>HHHHHHENLYFQSMAVSPSPLRIFTAGGTIDKDARLEENGLVVGDPFVAEVLKTARLAGAVSIVALSRKDSLDFTEADREAIGRAVGQAVEDHILLTHGTDTMVETARYLGGLPELAGKTVVLSGAMVPGRVGGSDAAFNIGFACAAALMLAPGVYIAMHGKVFDPAKTRKNRGLGRFEPIDDQE[4x]

L‐Asparaginases (ASNases) catalyze the hydrolysis of L‐Asn to L‐Asp and ammonia. In contrast, the chain of ASNase from Rhodospirillum rubrum, reported here and referred to as RrA, consists of only 172 amino acid residues. RrA is homologous to the N‐terminal domain of typical bacterial class 1 ASNases and exhibits millimolar affinity for L‐Asn. Crystal structures of the wild‐type RrA, both with and without bound L‐Asp, as well as structures of several RrA mutants, reveal topologically unique tetramers.

Based on the previously published results for typical class 1 ASNases (Derst et al., 1994; Schalk et al., 2016), we tested two mutants, RrA(Y21A) and RrA(Y21F). RrA(Y21A) without added L‐Asp was disordered in the region of residues 22–26 and the active site contained a mostly disordered HEPES molecule contributed by the buffer. Solvent molecules occupied the space where the Tyr side chain is present in RrA(wt). In some cases, orthorhombic crystals with a doubled c axis were obtained, belonging to space group P212121. The a. u. for these crystals contained a complete tetramer. Although both were less active than RrA(wt), RrA(Y21F) is somewhat more active than RrA(Y21A), which is opposite to the results obtained for typical class 1 ASNases. While it is quite plausible that in RrA Tyr21 contributes to proton transfer from the primary nucleophile (Thr16), almost certainly its side chain also contributes to stabilization of the tetramer. In this role, substituting Tyr with Phe preserves this role better than the mutation Tyr → Ala.> TAPPEKPRRGWWR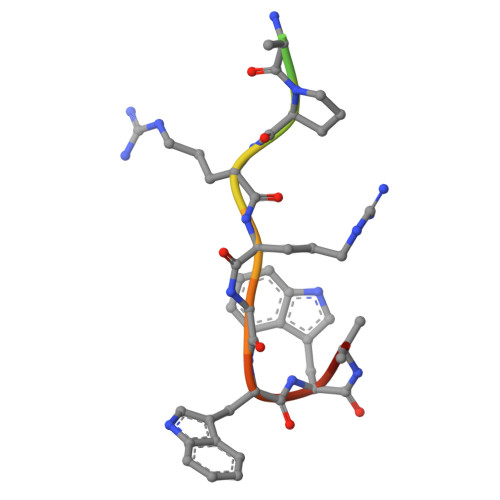R Here, we conduct a comprehensive functional analysis of the Antibiotic_NAT family of aminoglycoside acetyltransferases. AG resistance is primarily conferred by three classes of aminoglycoside-modifying enzymes (AMEs): phosphotransferases (APHs), nucleotidylyltransferases (ANTs), and acetyltransferases (AACs). AMEs permanently alter the AG substrate, preventing them from binding to their target, the A-site of the 16S rRNA in the bacterial ribosome. The fold typical of the Antibiotic_NAT family is evident in all structures, composed of 13 α-helices and 8 β-strands, and determined structures superpose with pairwise RMSD’s 0.8–1.0 Å between 197 to 266 matching Cα atoms.

We found that the Group 2 member AAC(3)-Xa, derived from an Actinomycetes, is limited in its AG specificity to the 4,6-disubstituted AGs kanamycin and tobramycin; the only other Group 2 member tested in our host E. coli was AAC(3)-IXa and did not convey any detectable AG resistance. As indicated by our AG susceptibility testing, the activity of AAC(3)-Xa is limited to tobramycin and kanamycin. To rationalize this strict specificity, we modeled the position of kanamycin into the active site of the apoenzyme structure based on the position of gentamicin bound to AAC(3)-IVa. This analysis suggested that gentamicin would not be accommodated due to the Tyr79 and Asp130 residues, which would clash with the 4”-OH group or the methylated 3”-amine of the corresponding AG substrate, respectively. Based on comparative analysis of the AAC(3)-Xa and AAC(3)-IVa•apramycin complex structures, Tyr79 would also introduce a steric clash with this AG in the AAC(3)-Xa active site. Notably, Tyr79, Asp130, Glu220, and adjacent active site residues are highly conserved in Antibiotic_NAT Group 2, suggesting these are critical determinants for restricting the specificity of these enzymes. In contrast, the AAC(3)-Xa enzyme exists as a monomer in solution despite forming a dimer in the crystal lattice. Representatives of Antibiotic_NAT Groups 2 and 4 were the most restricted in their specificity, and this was reflected in more constrained and smaller active sites, as revealed by the structures of AAC(3)-IIb and AAC(3)-Xa.

>DYKDDDDKMDETELLRRSDGPVTRDRIRHDLAALGLVPGDTVMFHTRLSAIGYVSGGPQTVIDALLDVVGPTGTLLVTCGWNDAPPYDFTDWPPAWQEAVRAHHPAFDPRTSEAEHANGRLPEALRRRPGAVRSRHPDVSLAALGASAPALMDAHPWDDPHGPGSPLARLVALGGRVLLLGAPRDTMTLLHHAEALAQAPGKRFVTYEQPIEVAGERVWRTFRDIDSEHGAFDYSSAVPEGQDPFAVIVGSMLAAGIGREGFVGAARSRLFDAAPAVEFGVRWIEEHLNRDR[2x]> MHHHHHHSSGRENLYFQGGKKQPSLHYTAAQLLEKGVLVEIE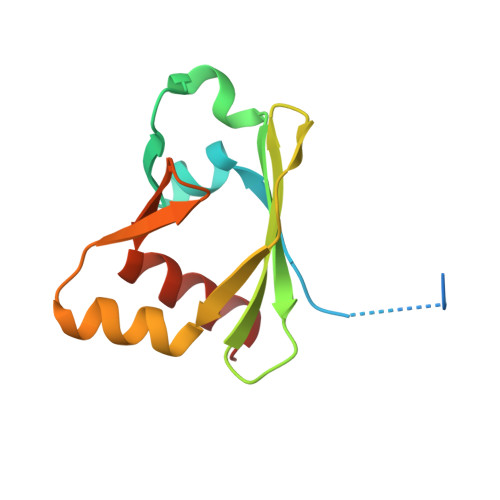DLPASHFRNVIFDITPGDEAGKFEVNAKFLGVDMERFQLHYQDLLQLQYEGVAVMKLFNKAKVNVNLLIFLLNKKFLRK> MIEETAKKVKELGFKKAGLLATTGTIVSGVYEKEFSKYGVEIMTPTEDEQKDVM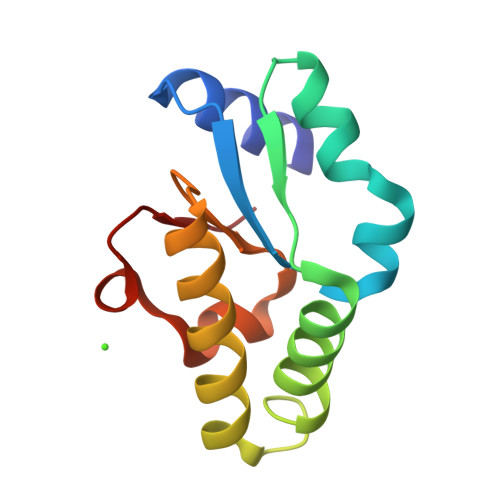RGIYEGVKAGNLKLGRELLLKTAKILEERGAECIIAGCTEVSVVLKQDDLKVPLIDP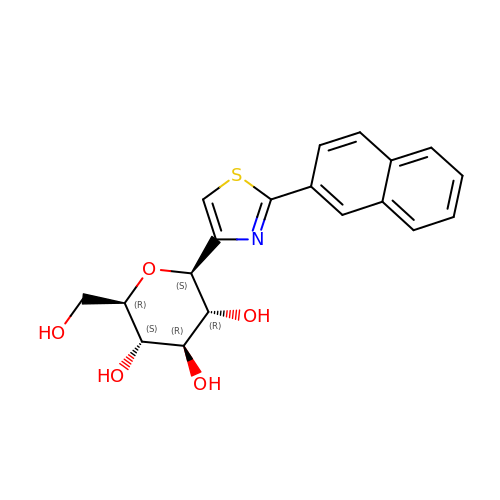(2~{R},3~{S},4~{R},5~{R},6~{S})-2-(hydroxymethyl)-6-(2-naphthalen-2-yl-1,3-thiazol-4-yl)oxane-3,4,5-triol | C19 H19 N O5 S | FZKCJLOBYMCTSR-SFFUCWETSA-N>[2x]MRGSHHHHHHGSNHYDFQGRSAIITGGAQGFGYAVAERLLQGKAKVVLWDMDDKALAEARAKLEPLGNVETVRVDISDQSDVQQAIEATEKLTQSIDILVHSAGIAGQNNPVADYSPEEWRRVIDIDLNGAFYVNQVVVQRMIAQNYGRIVNIASIAGKEGNPTASAYSAAKAGMIALTKSLGKETATRNIAVNAITPAAAQTRILEQCTQAHIDYMLSKIPRARFV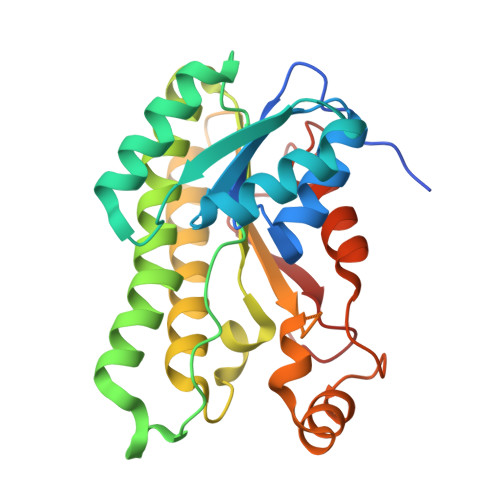KVEELAAMVAWLVSEENSFTTASVFDLSGGRATY> MLYIDEFKEAIDKGYILGDTVAIVRKNGKIFDYVLPHEKVRDDEVVTVERVEEVMVELDKLEHHHHHH;> MLKDFGKKIKSLRLEKGLTKEAVCLDESQLSTRQLTRIESGQSTPTLNKAVYIAGRLGVTLGYLTDGE

Within S. pyogenes, Prx functions to inhibit the quorum-sensing receptor-signal pair ComRS, the master regulator of natural competence, or the ability to uptake endogenous DNA. ComR is a quorum-sensing receptor and a transcription factor that belongs to the Rgg subgroup of the RRNPP protein family, many of which regulate virulence in pathogenic Streptococcus species. ComR is a monomer that contains a DNA-binding domain (DBD) packed against a tetratricopeptide repeat (TPR) domain. Specifically, Prx binds directly to the apo-form of ComR preventing DNA binding in vitro and acts as a repressor of the S. pyogenes competence regulon in vivo.

Despite not being able to obtain an X-ray crystal structure of Prx in complex with full-length ComR, we were able to cocrystallize Prx with the DBD of ComR. DBD:Prx cocrystals were obtained with both purified minimal DBD bound to Prx and after in situ proteolysis with full-length ComR complexed with Prx. In the case of the proteolysis experiment, full-length ComR was cleaved within the linker region that joins the DBD to the TPR. The crystals grew in similar conditions and both diffracted to 1.65 Å and 1.60 Å, respectively. The obtained complexes are nearly identical except for differences in space group (P212121 and P41212) and their cloning and protease digestion artifacts. Analysis of the DBD:Prx complex interface reveals that Prx directly interacts with the DNA-binding surface of ComR. The interaction is highly electrostatic in nature, with Prx using a large negative surface consisting of conserved acidic residues to complement the conserved positive DNA-interaction face of the ComR DBD. At this interface, Prx makes several hydrogen bond and salt-bridge contacts with key residues in the DBD that are critical for interaction with DNA. If the DBD:Prx complex is aligned to apo-ComR using the DBD, we observed that Prx is unable to interact with the DNA-binding residues of ComR due to a large steric clash as this surface is held tightly against the TPR domain. As such, to bind ComR, Prx must induce a conformational change in apo-ComR to interact with the DBD.> QSCAT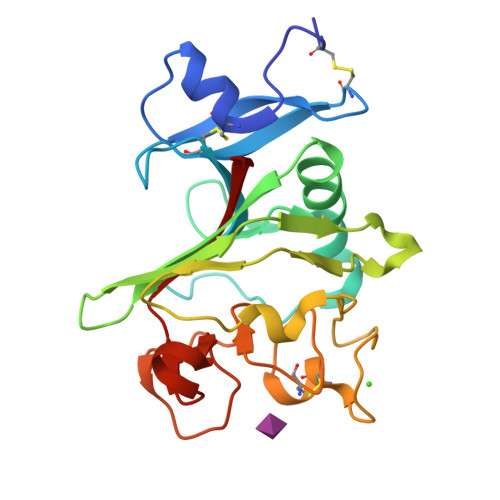GPRNCKDLLDRGYFLSGWHTIYLPDCRPLTVLCDMDTDGGGWTVFQRRMDGSVDFYRDWAAYKQGFGSQLGEFWLGNDNIHALTAQGSSELRTDLVDFEGNHQFAKYKSFKVADEAEKYKLVLGAFVGGSAGNSLTGHNNNFFSTKDQDNDVSSSNCAEKFQGAWWYADCHASNLNGLYLMGPHESYANGINWSAAKGYKYSYKVSEMKVRPA> QNNTDYPFEANNPYMYHENPMEEGLSMLKLANLAEAALAFEAVCQKEPEREEAWRSLGLTQAENEKDGLAIIALNHARMLDPKDIAVHAALAVSHT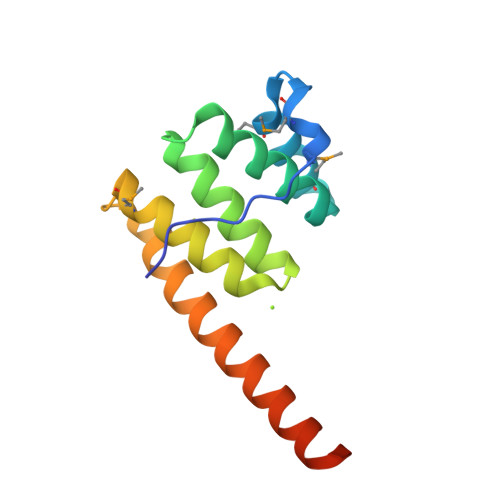NEHNANAALASLRAWLLSQPQYEQL> MSIVTKSIVNADAEARYLSPGELDRIKAFVTGGAARLRIAETLTGSRETIVKQAGDRLFQKRPDIVSP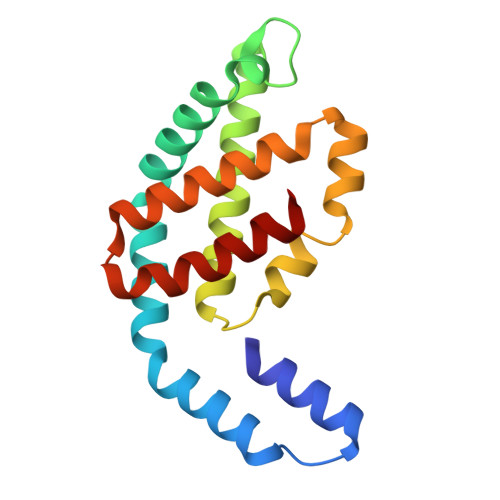GGNAYGEEMTATCLRDMDYYLRLVTYGVVSGDVTPIEEIGLVGVREMYRSLGTPIEAVAQSVREMKEVASGLMSSDDAAEASAYFDFVIGKMS>[2x]MGLNIGDLLGSTPAKDQGCSRTC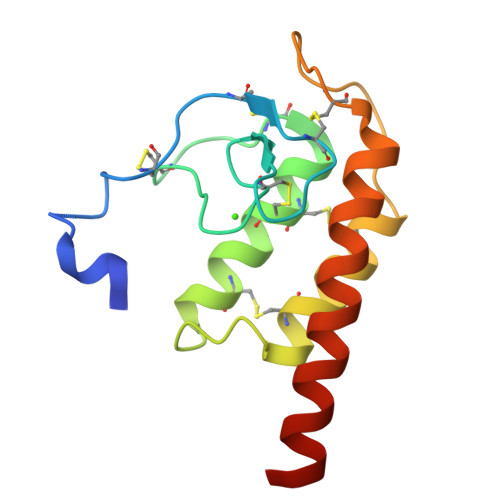ESQFCTIAPLLRYGKYCGILYSGCPGERPCDALDACCMVHDHCVDTHNDDYLNTMCNENLLSCIDRVSGATFPGNKCNVGQTASVIRGVIETAVFAGKILHKRDDGQ Group 1 and group 2 chaperonins are two distinct classes of chaperones that exist in diverse organisms to assist with protein folding in an ATP-dependent manner. In both chaperone groups, each monomer is comprised of three domains: an equatorial domain, an intermediate domain, and an apical domain. The equatorial domains contain the ATP binding site, the intermediate domain serves as a hinge connecting the equatorial to the apical domain, and the apical domain is involved in substrate binding. The overall structure of PfCpn60 represents a typical group 1 chaperonin, with a sevenfold symmetrical cylinder consisting of two back-to-back stacked rings composed of seven subunits.

In order to understand its mechanism in P. falciparum, we report the first crystal structure of P. falciparum Cpn60 (PfCpn60) bound with ATP, which reveals the large conformational dynamic of the apical domain relative to the intermediate and equatorial domains. No crystals were grown from WT-PfCpn60 probably due to the structural heterogeneity caused by the fast hydrolysis of ATP in WT-PfCpn60 which occurs in the matter of seconds. Comparatively, it is estimated that the D474A mutation slows hydrolysis to a rate of around 40 min. One heptameric ring was found per asymmetric unit of the PfCpn60 structure. A second heptameric ring in an adjacent asymmetric unit that is related by twofold crystallographic symmetry results in a tetradecameric complex with the rings stacked back-to-back, as observed in the other Cpn60 structures. The seven subunits in the asymmetric unit are in slightly different conformations and differ from the closed and opened conformations typically observed for other Cpn60 molecules. The superimposition of the current structure with the closed and opened conformation of TtCpn60 (using the equatorial domain) confirmed that the conformation of the PfCpn60 structure is a unique ATP-induced conformation distinct from both the closed and open conformation. In the current structure, the apical domains of subunit B, C, and F are much more mobile (weak electron density and high-temperature factors) than those of subunit A, D, E, and G, due to less interaction with other symmetry-related molecules. One unique feature of PfCpn60 that impacts intra-ring subunit-subunit interactions is the extra 27 residue insertion (residues 513–539, α15–α16) that forms an extended α-helix loop and contacts the left-handed intra-ring subunit. The inter-ring subunit-subunit interface buried area of 683 Å2 in PfCpn60 is much larger than the buried area of ~ 200 Å2 in other Cpn60 structures, due to the extra 27 residue insertion in PfCpn60.

>MTGKGKDIIYGNECRNELLKGILTVSDVVKLTLGPRGRNVLLEKEYGSPLIINDGVTIAKQISLKDRKKNNGVKLMQESTQISNDKAGDGTSSTALMTATITKKGIEQVNRNHNPIPIQRGIQLASKMIIEKIKSLSTPIKTYKDILNIATIASNNDVHMGQIIANAYDKLGKNAAIILDDNADINDKLEFTEGYNFDRGIINPYLLYNENKDYIEYSQVSTLITDQNIDNIQSILPILEIFAKNKQPLCIIADDFSNEVLQTLIINKLKGAIKVVPIRAPSFGDRRKDYLKDLCIVTNSKYISADVGLDLNNLHNQMSSFDNNYLSLLGSANTLIVKKDRTSLITKEEYKKEIDERINVLKKEYEETTSKYDKEKLNERIAALSGGIAKILIGGNSETEQKERKFKYEAATNAVKSAIDIGYVPGGGVTYLEIIKSNFIQEIHKKIEEDLQISSNNDEKKYLELIGNLESEMELQKMGANIVVSSLDVITKQIADNAGVNGDNVVKIILNSKDKYGFGYDVNTNKFVNMVEKGIIDSTNVIISVIKNSCSIASMVLTTECMMVDHEK[7x]>[2x]RRTRRDEDDLEQYLDEKILRLKDEMNIAAQLDIDTLNKRIET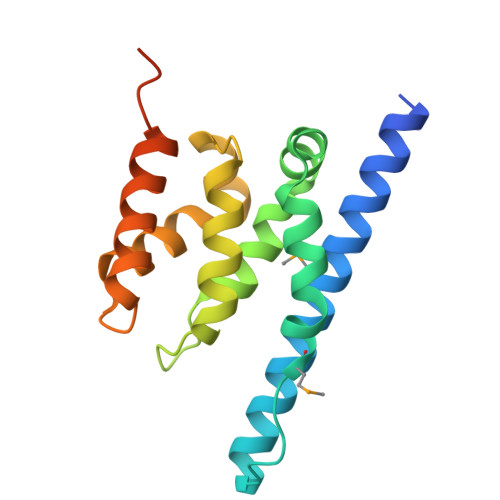GDTSLIAMQKVKLLPKVVSVLSKANLADTILDNNLLQSVRIWLEPLPDGSLPSFEIQKSLFAALNDLPVKTEHLKESGLGRVVIFYTKSKRVEAQLARLAEKLIAEWTRPIIGASDNYRDKRIMQLEF>[4x]RMEIVKIPVVVHVVWNEEEENISDAQIQSQIDILNKDFRKLNSDVSQVPSVWSNLIADLGIEFFLATKDPNGNQTTGITRTQTSVTFFTTSDEVKFASSGGEDAWPADRYLNIWVCHVLKSEIGQDILGYAQFPGGPAETDGVVIVDAAFGTTGTALPPFDKGRTATHEIGHWLNLYHIWGDELRFEDPCSRSDEVDDTPNQADPNFGCPSYPH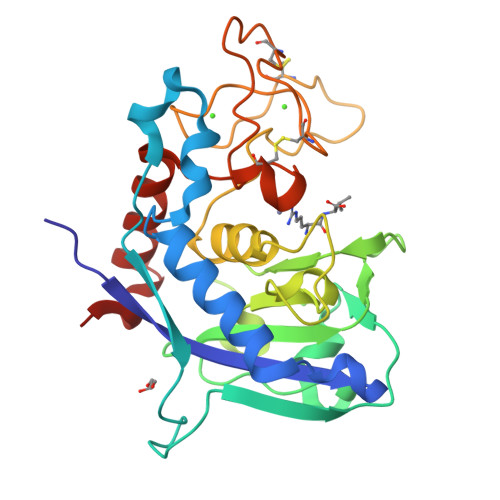VSCSNGPNGDMFMNYLDYVDDKCMVMFTQGQATRVNACLDGPRSSFLA(2S)-2-amino-4-{[(1Z)-{3-hydroxy-2-methyl-5-[(phosphonooxy)methyl]pyridin-4-yl}methylidene]amino}butanoic acid | C12 H18 N3 O7 P | 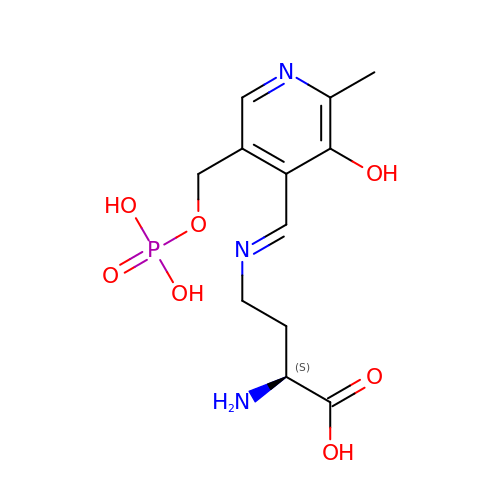BBWBZEWRKQXPMM-YXBHYIBOSA-N RNA uridylation is catalyzed by a class of template-independent terminal ribonucleotide transferases (TENTs) or terminal uridylyl transferases (TUTases). In Arabidopsis, HEN1 SUPPRESSOR1 (HESO1) and URT1 (UTP:RNA uridylyltransferase) act cooperatively on unmethylated miRNA uridylation to trigger their degradation. In addition, URT1 uridylates a subset of mRNAs with short poly(A) tails and is negatively involved in post-transcriptional gene silencing. It consists of two canonical globular domains, the catalytic domain and the central domain, separated by a large catalytic groove where RNA substrate usually binds.

To further explore the URT1-mRNA recognition, we co-crystalized the URT1 (410–764) with a 5′-AAAU-3′ RNA stretch and obtained their complex structure at 1.8 Å resolution. In this structure, RNA bound URT1 in a canonical way with 3′-U sitting in the UTP binding site (+1 position) of URT1, and three other adenines sequentially occupied the 0, –1 and –2 RNA-binding positions along the catalytic groove. Unexpectedly, different from our and other previous researches in which the structures of apo- and RNA-bound forms of TUTases are basically the same, URT1 experienced a large conformational rearrangement upon the RNA binding, with its entire catalytic domain rotated by ∼30° from its original position in apo-form (open state) toward to the central domain, about the joint region of these two domains, to form a more compact structure (closed state). In the URT1–AAAU complex, the 0 nucleotide-binding position was occupied by an adenine (A0) representing the 3′ extremity of the mRNA poly(A) tail. Among the URT1 residues surrounding A0, N552 provided the specific contact with the adenine by forming a hydrogen bond between its side-chain group and purine N3, while V532 made a hydrophobic interaction against the base. Unlike the +1 and 0 nucleotide-binding sites, URT1 possesses a group of less conserved residues for RNA recognition at the –1 position, where the protein–RNA interactions are dominated by hydrophobic stacking. The adenine at this site (A–1) was perfectly sandwiched by the side-chain groups of Y592 from the central domain and L527 from the catalytic domain. At the –1 position, we noticed that both the side-chains of L527 and Y592 stacked exactly with the pyrimidine ring of A–1 but not its imidazole ring. Clearly, our results showed that both A2U and A2C are weakly tailed by URT1 whereas A2G is properly tailed in a pattern very similar to poly(A) but with somewhat lower efficiency. These results are consistent with our above speculation and suggest a conclusion that L527 and Y592 help URT1 to establish a preference for purine over pyrimidine at the –1 nucleotide-binding position. More strikingly, the R531 from the SSL loop largely re-orientated its side chain with the end group of side chain shifted by 16.9 Å to form a 2.6 Å hydrogen-bonding interaction (salt bridge) with D700 from the central domain.

> MGHHHHHHMGQRLLGQKARMVKMYMACRNDIHRYDATFIAIYKSLIPAEEELEKQRQLMAHLENLVAKEWPHAKLYLYGSCANSFGFPKSDIDVCLAIEGDDINKSEMLLKLAEILESDNLQNVQALTRARVPIVKLMDPVTGISCAICINNVLAVVNTKLLRDYAQIDVRLRQLAFIVKHWAKSRRVNETYQGTLSSYAYVLMCIHFLQQRRPPILPCLQEMEPTYSVRVDNIRCTYFDNVDRLRNFGSNNRETIAELVWGFFNYWAYAHDYAYNVVSVRTGSILGKREKDWTRRVGNDRHLICIEDPFETSHDLGRVVDKFSIRVLREEFERAARIMHQDPNPCAKLLEPYIPEDNNGQGHN Here, we show that Pseudomonas aeruginosa OprC is an outer membrane, TonB-dependent transporter that is conserved in many Proteobacteria and which mediates acquisition of both reduced and oxidised ionic copper via an unprecedented CxxxM-HxM metal binding site. As indicated by the successful structure solution, OprC contains a single bound copper and shows the typical fold of a TBDT, with a large 22-stranded β-barrel occluded by an N-terminal approximately 15 kDa plug domain that, like in other TBDTs, completely occludes the lumen of the barrel. The copper binding site comprises residues Cys143 and Met147 in the plug domain and His323 and Met325 in the barrel wall. The CxxxM-HxM configuration, which coordinates the copper in a tetrahedral manner, is highly unusual and has, to our knowledge, not been observed before in copper homeostasis proteins.

C143A has no bound copper even after incubation with 10 equivalents Cu(II), suggesting that this residue has a crucial role. While OprCWT and most single alanine mutants can be (partly) loaded via Cu(II) incubation, this is not the case for the C143A mutant. We hypothesised that removal of the cysteine could lead to much lower affinity for Cu(II), so that after SEC, nothing remains bound. To provide support for this, we determined the crystal structures of the OprC C143A mutant cocrystallised with Cu(II) or silver Ag(I). For each crystal, datasets were collected at 8,800 eV and 9,175 eV to distinguish between both metals. Bound copper is expected to give a strong anomalous peak only at 9,175 eV (which is above the copper K edge at 8,979 eV), while bound silver will give comparable peaks at both energies (the silver L-III edge is at 3,351 eV). For C143A cocrystallised with Cu(II), no anomalous peaks are visible at both energies, showing that Cu(II) binding is indeed abolished. All 4 residues in the OprC binding site contribute to copper binding, but not to the same extent and, in some cases, not equally for both copper redox states. This is illustrated by Cys143, which is essential for high-affinity Cu(II) binding but dispensable for Cu(I).

>MEKRMSTQQRAAGNACPTAAFSFDPARLAQRRRWAGAFAALCGLALSPSALLAEEHSQHQDHAVELAPSVVTGVAQSSPLTIVTNPKEPRQPVPASDGADYLKTIPGFAVIRNGGSNGDPVLRGMFGSRLNILTNGGMMLGAAPNRMDAPTSYISPETYDKLTVIKGPQTVLWGPGASAGTILFEREPERFGELGSRVNASLLAGSNGRFDKVLDAAAGNRLGYLRFTGNHAQSDDYEDGAGNTVPSRWKKWNGDVAVGWTPDEDTLIELTAGKGDGEARYAGRGMDGSQFKRESLGLRFVKSNVSDVLEKVEAQVYYNYADHIMDNFRLRTPDPSSMMPMPMASQVDRRTLGGRLAATWRWDDFKLVTGVDAMRNEHRARGSKYDMMTDYYTDADQFPWSKDAVFHNYGAFGELTWFAAERDRLIGGLRLDRASVKDYRQTLKSGHMGHAMANPTANDTRADTLPSGFVRYEHDLADSPTTLYAGLGHAERFPDYWELFSPKRGPNGSVNAFDKIKPEKTTQLDFGLQYNGDKLQAWASGYVGVVQDFILFSYREGMMGSSTQATNVDARIMGGELGASYQLTGNWKTDASLAYAWGKNSSDDRALPQIPPLEARFGLTYEEGDWSAGSLWRVVAPQNRIARDQGNVVGKDFDKSAGFGVFSLNGAYRVTRNVKLSAGVDNLFDKDYTEHLNKAGDAGFGFSANETVPEPGRTFWTKVDFSF[2x]>MQEKQLKAIQNKIASWIKEIESGFIDELFSKIGPSKMLRSKLMLALLNEKTDAILLDKALNLCTIVEMIQTASLLHDDVIDKATMRRKLPSINALFGNFNAVMLGDVFYSKAFFELSKMGELIAQALSNAVLRLSRGEIEDVFVGECFNSDKQKYWRILEDKTAHFIEASLKSMAILLNKDAKIYADFGLNFGMAFQIIDDLLDITQDAKTLGKPNFSDFKEGKTTLPYLLLYEKLNQHDQGLLISYFKQDSHEI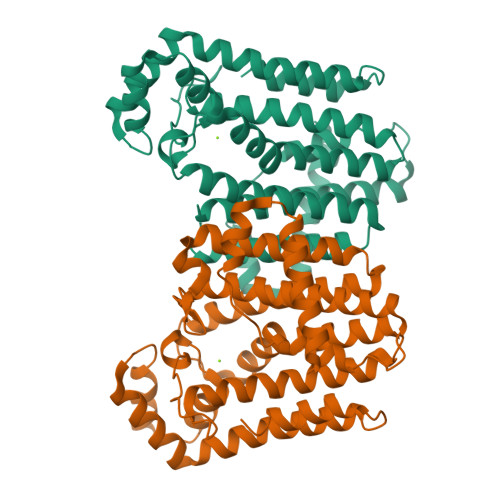IEWTKEKFKQYGIIEETLKTAQVYSKKALEAIKGENNLILEKLAQDVISRTFLEHHHHHH[2x]> METKINRKLLYPPIDNFNYGNTHHNNNKQPNINHEEIPSGITSDGNYSWFTKENEIFFYDLNNGKRITTFCFVVENSIECSVTAVGEIIVEDQIFIVVALKGGNSTSLKVLDIQTGDTLKTLDTTPLSTITYIKQLYRESKFSKAQADLIRNIKTPLALGIQNSCQVIIVDIYFNLREQFLSSNQLILQDITNYDYKHFFNNKTNNLVPYFILGGDQLFNGNSYKFEYPAGKHSSEGYLVEDRNGITQQNLKSKLQHQYPQQQQQQQQQQQQQQTNQFTQLDVTSIEYIESLRMIAIGYSIGTFQLFSSNNFKLYYCSPAREVGLHSSVSHLENKQSPVTNFLYQELEDDDTSSVSHLWIGRGSKNNKSSNNNISIILYKLEFDLQLSPDSSKTINNLISLTQNVDTPIDITKINQTNSQTNQFGEILLMSYLYQNKDLKLNNGIIPKSKSIFIYQFIENGTIKIEIKLFDLFLLERHGINYSSNSQQHWLHSIKLDDENGNFKNNGYHSIWIDQQSVLNNVLYQLENNNSKVFLSKEDQYQTSGSNSGSGSDNFDDNYENFEENKLNLTIYHPNFKFKLLSFSTIDNIDYLSPKERLVYELSNKGAILFESSTLLNSVYVKFVESNIFPFYKSDQQQQRNDLLIFSLNNNLISIVKDYILNYKSSNAKLILESFWSHFQTLNRNFGLSEIYSKLNSDTPKLLELVYVKITDLVRIFKSLADRYIQENLNKLNSNDMIIDGGGGGGGSNSNSNLNSNSNLLPDTLKIKIDQAINIARFIEILKWSLYFGLFKPSTLNDMESVRNYTIQKRKIIKEKLTIEMGNIGRTNQYLSDRLLIDLFYSNIDLSSSTSTTTTTTTTTTDGNQIMSSYPPHNSQTMKSFFKIFESSQQFTKKISVLFYLLIDLELTDLNGGNGSNGKSLHQSETLKSFFGSFHISSNYYSFIMGIWKLDSYLLKSQDQMNIDDDDDDDEDATNRENNSNLIDEDIKSAFTLLNSSKVTKKYLYPILARFYSFGFKNYAQLLMKGFNFQPQTPDEAQLYVRILLSNHSILEAILFQRSFRNRLQDQLTIDSIERLLFSIFNYTFNLKKLDLILNMSLDEIEEQVFLHFLFKMKASSLISLYYIKRGRIPEACKVNRYYQSTRVNGDVFDGHDTINHLLLNYEQSLPLIQRPIHFNITNESQDKPKQQPQSQQQQQQPQPQQFLNSEEDNIPLLPKSISKVNLVPPQSFIQKPIVMPSPIPKLYNDSLYLSSTLSTAPISNLEILTKKSNEEQQERLLIQQRLAQQEKELQEQQRIKKEFEDQQEKLLDFQRQQELLQHQMEVHSQLLLQQKQQQQQQQKQIKEQEYEEYDEEYEEEEEEQVATSNKSSLDMIFPTMVTTTSTTTSSPNLSVASGSTPQGSPLKSALKSGGSAKKTTNVRFKDSLNREYPIPKLKKRGMPDSDDDDDDDDENYDSDDDDDDDEDSEFEDIYKIDSNEDEEEDEEDEEEEDDDSAVVHDDDELDDQQASQAQQFLQNQKHQKLLQQQQQQQQQQQQQQQQQQQQQQQQQQQQQQQQHETDDTEEELEDDIVEEDDDSEEDRFKDFERPKHGGKEPPKFSTYSGLQPSKQQQQKFLSPQDDDDYDEEDEEDDQSYDDDDDGEEEDDGNYRVPTQQFMRQPIVNSSSSGGTQDEPMEIGSSSDEDNSQIVKNQYNYNNEEDNDEDEQEDDNEEEQEEDEEEEEDSPKQPKRVVAHKPLPKVQFNNNDEEEQQQQQQQQQQQQQQQQQQQQQQQQQQQKEEEEEEEEEEEEKKMNESDESGGEISKNENSSDDDSDNDQFNSPFTNQFLSKTSGNTSGQSIDFDQDEKYSTPTDKGSNNNDTTVDSDIFQSQQSDSSFVQSQENESLKKSDENLSTFNDLNNSILSNISSQQPQEDDEKFQELEGDTNNNNNNNNNNNNNNNNNNNTDEVMGDEEKNDNQNVEMENTEQDKKDSPFQEIEDDESIINSQQKEESDVEGKSNDQSLETSIHQKVEDKQMDDDDDEKSNNQNEENVQPTQEKQDEQEPEEQEEQEKQPEEEEEEEEKVKEIEQQEEEEEEPKEEQSEEEEEEQPEEEQPEEEQTKEEQPGEEQPGEEEEEPEEEEEEKEPEEEEEEEKEMEEDEEEKEDEEEEKEDTPKKQPIVPISTRPSRQSKTDGIAKTLSIA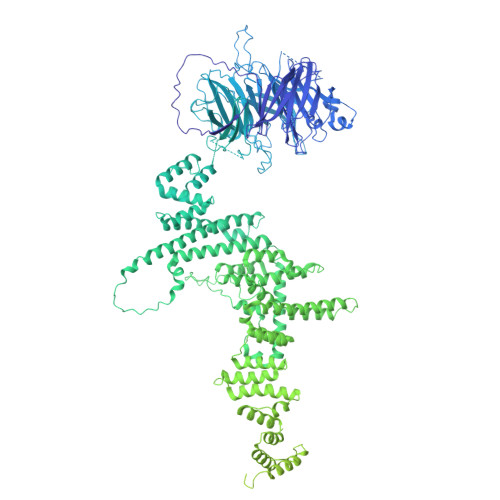EMRRGEKDKKKQLAPQKPTSKLKPKVQAATKPKKTKKASKK> MAGIFDRIAGASGADETELTAEPMALDDGMDGEQPAMSANIQVDERRTPQRVREAVQEMLKYGLLEESHKPNLYRSALTNIEVVDRILEPLDLAMGVDEVRGLVFVTVRQGEVAEQDDWSHPLVRRQRLN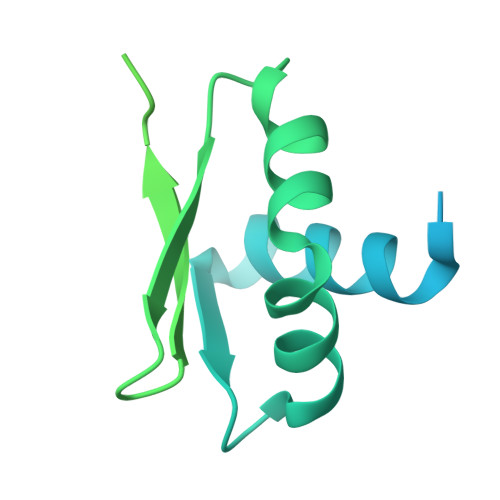LEQSLLIAILRQHFIAYEQESGTGASQALVAVDELIPQLQVYLGELGSEAKERNRIITLLDQLKGHGLVSALDAHDRVIIRPIITHLANPENLQALVVWLREQVEGAVTPAAGGEEDEA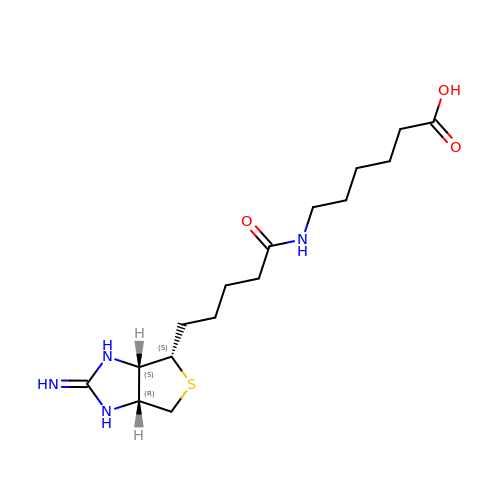6-({5-[(2E,3aS,4S,6aR)-2-iminohexahydro-1H-thieno[3,4-d]imidazol-4-yl]pentanoyl}amino)hexanoic acid | C16 H28 N4 O3 S | IAJKFHSLWUNBII-HUBLWGQQSA-N3-ethoxy-6-{2-[1-(6-methylpyridazin-3-yl)piperidin-4-yl]ethoxy}-1,2-benzoxazole 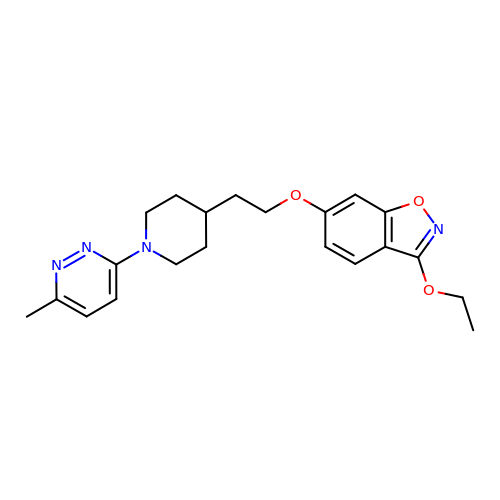| C21 H26 N4 O3 | DKSVBVKHUICELN-UHFFFAOYSA-N>LEEEDVICDGCNGPVVGTRYKCSVCPDYDLCSVCEGKGLHRGHTKLAFPSPFGHLSEGFS[2x]

Intriguingly, the autophagy adapter p62/SQSTM1/Sequestosome-1 was recently reported to recognize N-degrons, the N-end rule substrates of the well-characterized UPS, and where ultimately these substrates are delivered to ALS8,9. p62 is a key selective autophagy adapter that plays a role in the degradation of various cellular constituents such as misfolded proteins and their aggregates, malfunctioning organelles, and invading pathogens. Intriguingly, it was recently reported that the central ZZ-domain in p62 plays a critical role in the recognition of N-terminal arginylated BiP/GRP78 by the Arg-tRNA transferase ATE1. Here, we present the high resolution structures of the ZZ-domain of p62 in complex with 8 different N-degrons including type-1 and type-2, and subsequently identify key determinants involved in the unusual recognition.

However, an understanding of the manner by which the ZZ-domain binds to type-2 substrates is problematic since there is no deep hydrophobic pocket in the ZZ-domain, which is known to be involved in the recognition mode for type-2 N-degrons. Therefore, we determined the structure of the ZZ-domain in complex with a variety of N-degrons comprising three type-1 N-degrons and five type-2 N-degrons. As described for the R-BiP complex, two aspartic acid residues, Asp129 and Asp149, bind to the α-amino group, and Asp147 forms a hydrogen bond with the first peptide bond, which means that these interactions are conserved in all different N-terminal residues. However, the side chain of the N-terminal residue of the N-degron is recognized differently. Furthermore, the hydrophobic side chain of Ile127 guides the orientation of the side chain of the primary residue. Therefore, relatively small and branched hydrophobic residues at the primary position might provide very weak (or no) interactions with the binding patch of the ZZ-domain.>[2x]PKALIVYGSTTGNTEYTAETIARELADAGYEVDSRDAASVEAGGLFEGFDLVLLGCSTWGD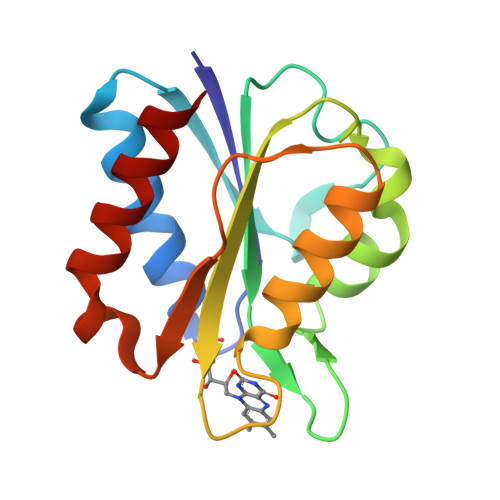DSIELQDDFIPLFDSLEETGAQGRKVACFGCGESSYEYFCGAVDAIEEKLKNLGAEIVQDGLRIDGDPRAARDDIVGWAHDVRGAI> RLTERAQRVLAHAQEEAIRLNHSNIGTEHLLLGLMKEPEGIAAKVLESFNITEDKVIEEVEKLIGHGQDHVGTLHYTPRAKKVIELSMDEARKLHHNFVGTEHILLGLIRENEGVAARVFANLD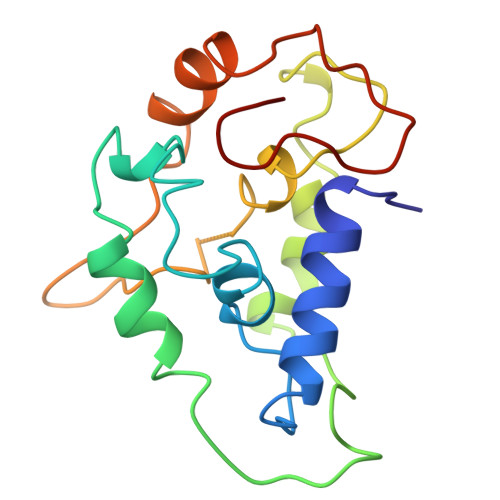LNITKARAQVVKALGNPEMSNKNAQASKSNNTP>MVLYFIGLGLYDERDITVKGLEIAKKCDYVFAEFYTSLMAGTTLGRIQKLIGKEIRVLSREDVEQNFENIVLPLAKENDVAFLTPGDPLVATTHAELRIRAKRA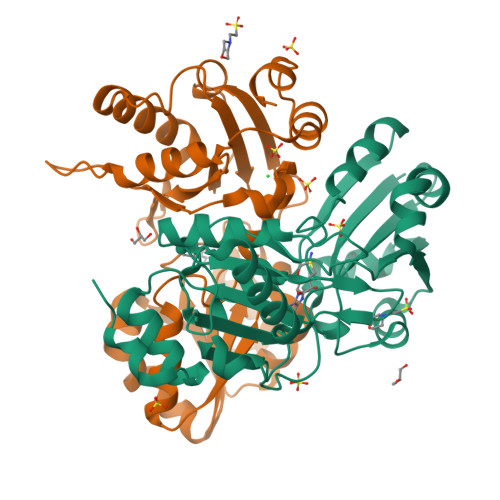GVESYVIHAPSIYSAVGITGLHIYKFGKSATVAYPEGNWFPTSYYDVIKENAERGLHTLLFLDIKAEKRMYMTANEAMELLLKVEDMKKGGVFTDDTLVVVLARAGSLNPTIRAGYVKDLIREDFGDPPHILIVPGKLHIVEAEYLVEIAGAPREILRVNV[2x]> MKHHHHHHMKQNSPLDEENLTQENQDRGTHVDRGLASANVDFAFSLYKQLVLKAPDKNVIFSPLSISTALAFLSLGAHNTTLTEILKGLKFNLTETSEAEIHQSFQHLLRT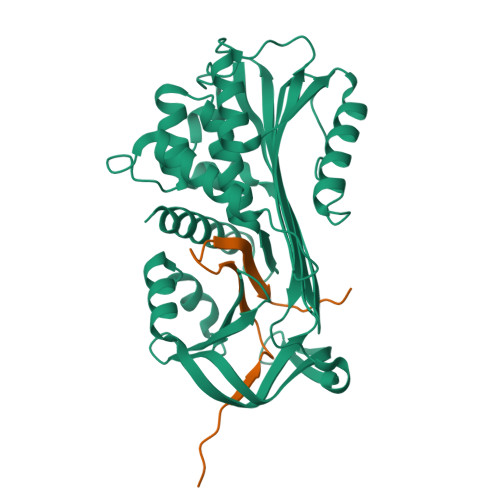LNQSSDELQLSMGNAMFVKEQLSLLDRFTEDAKRLYGSEAFATDFQDSAAAKKLINDYVKNGTRGKITDLIKDLDSQTMMVLVNYIFFKAKWEMPFDPQDTHQSRFYLSKKKWVMVPMMSLHHLTIPYFRDEELSCTVVQLNYTGNASALFILPDQDKMEEVEAMLLPETLNRWGDSLEFREIGELYLPKFSISRDYNLNDILLQLGIEEAFTSKADLSGITGARNLAVSQVVHKAVLDVFEEGTEASAATAVKITLL;> SALVETRTIVRFNRPFLMIIVDHFTWNIFFMSKVTNPKQA2-[(~{E})-[2-methyl-3-oxidanyl-5-(phosphonooxymethyl)pyridin-4-yl]methylideneamino]propanedioic acid | 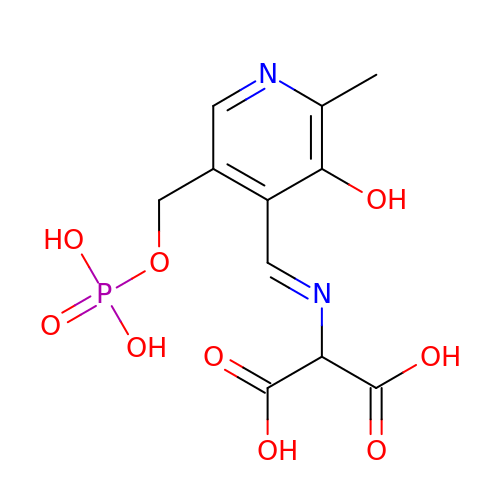C11 H13 N2 O9 P | NZWIGLKAYRQNJI-QLKAYGNNSA-N> FT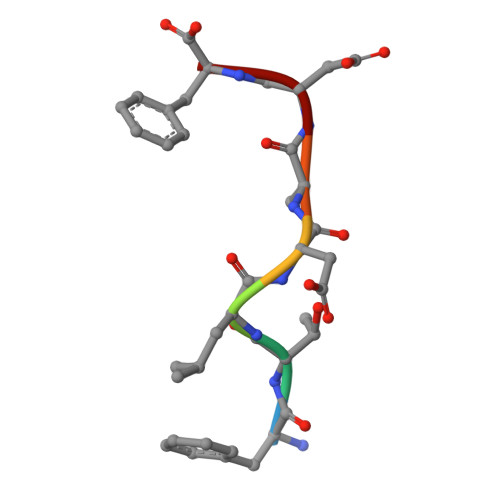LDADF> AAEFMKITILAVGKLKEKYWKQAIAEYEKRLGPYTKIDIIEVPDEKAPENMSDKEIEQ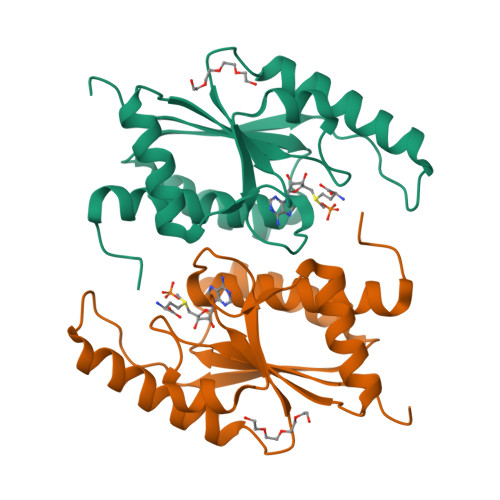VKEKEGQRILAKIKPQSTVITLEIQGKMLSSEGLAQELNQRMTQGQSDFVFVIGGSNGLHKDVLQRSNYALSFSKMTFPHQMMRVVLIEQVYRAFKIMRGEAYHK>[15x]EEATFTANFKDTDLKSFIETVGANLNKTIIMGPGVQGKVSIRTMTPLNERQYYQLFLNLLEAQGYAVVPMENDVLKVVKSSAAKVEPLPLVGEGSDNYAGDEMVTKVVPVRNVSVRELAPILRQMIDSAGSGNVVNYDPSNVIMLTGRASVVERLTEVIQRVDHAGNRTEEVIPLDNASASEIARVLESLTKNSGENQPATLKSQIVADERTNSVIVSGDPATRDKMRRLIRRLDSEMERSGNSQV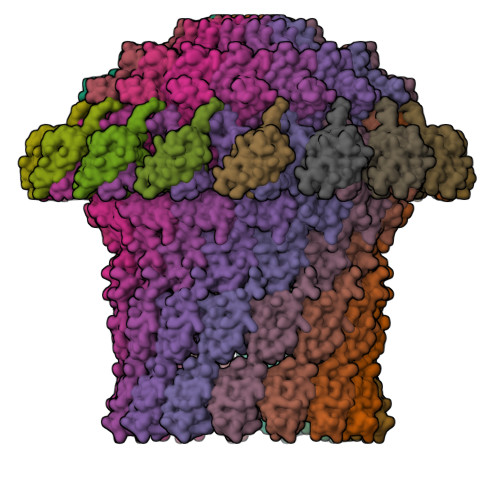FYLKYSKAEDLVDVLKQVSGTLTAAKEEAEGTVGSGREIVSIAASKHSNALIVTAPQDIMQSLQSVIEQLDIRRAQVHVEALIVEVAEGSNINFGVQWASKDAGLMQFANGTQIPIGTLGAAISQAKPQKGSTVISENGATTINPDTNGDLSTLAQLLSGFSGTAVGVVKGDWMALVQAVKNDSSSNVLSTPSITTLDNQEAFFMVGQDVPVLTGSTVGSNNSNPFNTVERKKVGIMLKVTPQINEGNAVQMVIEQEVSKVEGQTSLDVVFGERKLKTTVLANDGELIVLGGLMDDQAGESVAKVPLLGDIPLIGNLFKSTADKKEKRNLMVFIRPTILRDGMAADGVSQRKYNYMRAEQIYRDEQGLSLMPHTAQPVLPAQNQALPPEVRAFLNAGRTR;>[15x]CASHNENASLLAKKQAQNISQNLPIKSAGYTLVLAQSSGTTVKMTIISEAGTQTTQTPDAFLTSYQRQMCADPTVKLMLTEGINYSITINDTRTGNQYQRKLDRTTCGIVKA>[2x]GSHMLSEETIRVIKSTVPLLKEHGTEITARMFEL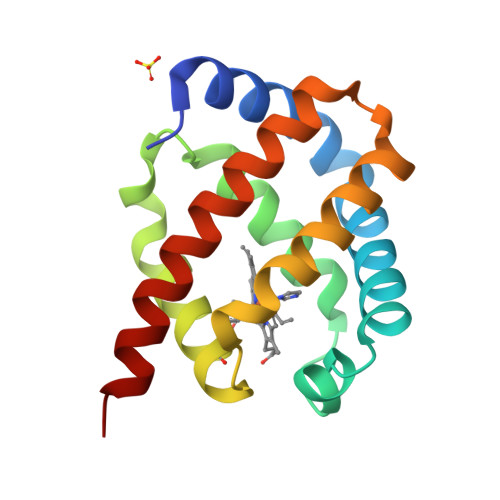LFSKYPKTKELFAGASEEQPKKLANAIIAYATYIDRLEELDNAISTIARSHVRRNVKPEHYPLVKECLLQAIEEVLNPGEEVLKAWEEAYDFLAKTLITLEKKLYSQP> GPLGSSIMKILLIGDSGVGKSCLLVRFVEDKFNPSFITTIGIDFKIKTVDINGKKVKLQLWDTAGQERFRTITTAYYRGAMGIILVYDVTDERTFTNIKQWFKTVNEHANDEAQLLLVGNKSDMETRVVTADQGEALAKELGIPFIESSAKNDDNVNEIFFTLAKLIQEKIDSN;>GPLGSNYNQLKEDYNTLKRELSDRDDEVKRLREDIAKENELRTKAEEEADKLNKEVEDLTASLFDEANNMVADA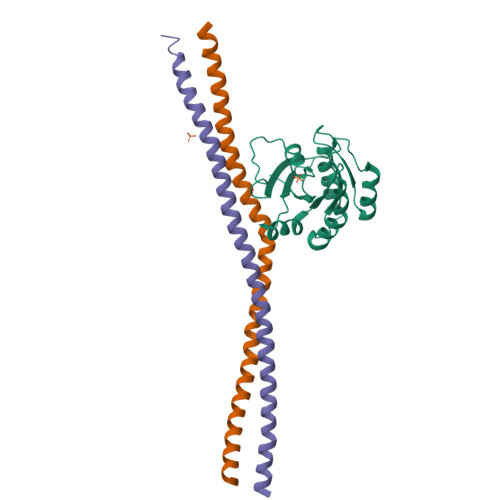RKEKYAIEILNKRLTEQLREKDT[2x]>MGIISYVKKLFKRPAGEIMRMSSGNIGVYKLDDSRVDYELARELYQNKNANYKLGSSFVRPIVNSTTGFMGVPHFQIEDEEAQYILDEFVLDNTSKMLKTHTDSLKQGDCYIWITREERENPLYPDKKVRLIYNFISPEEVKEIILDPTTKEPIAYILESQNEWTDLGENKRKAKVKQIITAESRFVEVEGDKIEGLEEGETPNVWGFIPIIHFKNEADETLKYGQSDIEPIEPLLKAYHDVMLHALKGSKMHSTPKLKLKLTDVASFLAHNFGVEDPVKFAKEGGKINLDGHEILFLNKDEEAEFVEVKSAIGDAKELLKLLFYCIVDVSETPEFIFGVHTPSALASVKEQMPIMVNKIRRKREQFTNSWQLLARMVLIMSSNSSGMKYSSYDVTIGWDEVNPRDDKELAETLEKVCCALDKALEGGFISEESTVNFLAQYIDTMSNYISDDPEREGEREKIIKTKMLKYRLDDSQGLNDESNEIEKEINKIKDNNGNG[12x]

Here, we reveal the extended and contracted atomic structures of an intact contractile-tailed phage (φCD508) that binds to and penetrates the protective S-layer of the Gram-positive human pathogen Clostridioides difficile. The virion can be divided into five distinct regions: the head, neck, tail, baseplate, and needle. Structures of purified φCD508 virions in both extended and contracted conformations were determined by single-particle EM of frozen-hydrated samples; the resolution ranged from 2.6 to 4.0 Å for the extended phage, and 2.9 to 4.2 Å for the contracted form.

At the base of the capsid sits a unique opening, centered on what would be a fivefold symmetry axis in a complete icosahedron; it is made up of 12 copies of portal protein gp45, forming an opening through which DNA is ejected from the capsid. Thus, there is a 5–12-fold symmetry mismatch between the capsid and the portal. (J) CryoEM density of C1 portal/capsid assembly showing the symmetry mismatch between the pentamer capsid vertex and the dodecameric portal. DNA density shown in yellow does not form interactions with any portal proteins.>NSSTASKTYNYVYSSDPSSLNYLAENRAATSDIVANLVDGLLENDQYGNIIPSLAEDWTVSQDGLTYTYKLRKDAKWFTSEGEEYAPVTAQDFVTGLQYAADKKSEALYLVQDSVAGLDDYITGKTSDFSTVGVKALDDQTVQYTLVKPELYWNSKTLATILFPVNADFLKSKGDDFGKADPSSILYNGPFLMKALVSKSAIEYKKNPNYWDAKNVFVDDVKLTYYDGSDQESLERNFT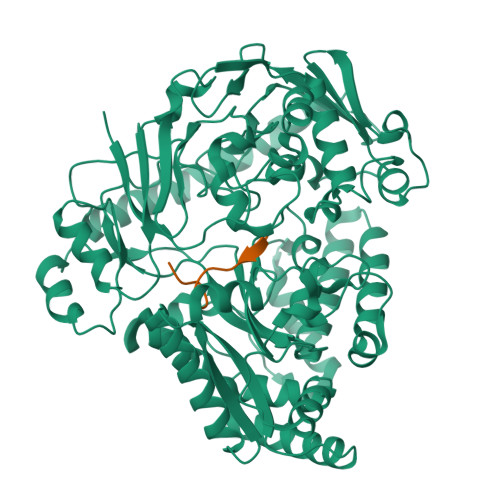AGAYTTARLFPNSSSYEGIKEKYKNNIIYSMQNSTSYFFNFNLDRKSYNYTSKTSDIEKKSTQEAVLNKNFRQAINFAFDRTSYGAQSEGKEGATKILRNLVVPPNFVSIKGKDFGEVVASKMVNYGKEWQGINFADGQDPYYNPEKAKAKFAEAKKELEAKGVQFPIHLDKTVEVTDKVGIQGVSSIKQSIESVLGSDNVVIDIQQLTSDEFDSSGYFAQTAAQKDYDLYHGGWGPDYQDPSTYLDIFNTNSGGFLQNLGLEPGEANDKAKAVGLDVYTQMLEEANKEQDPAKRYEKYADIQAWLIDSSLVLPSVSRGGTPSLRRTVPFAAAYGLTGTKGVESYKYLKVQDKIVTTDEYAKAREKWLKEKEESNKKAQEELAKHVK[2x];>[2x]PIVGGHEGAGV> VILPNNDRHQITDTTNGHYAPVTYIQVEAPTGTFIASGVVVGKDTLLTNKHVVDATHGDPHALKAFPSAINQDNYPNGGFTAEQITKYSGEGDLAIVKFSPNEQNKHIGEVVKPATMSNNAETQVNQNITVTGYPGDKPVATMWESKGKITYLKGEAMQYDLSTTGGNSGSPVFNEKNEVIGIHWGGVPNEFNGAVFINENVRNFLKQNIEDINFANDDQPNNPDNP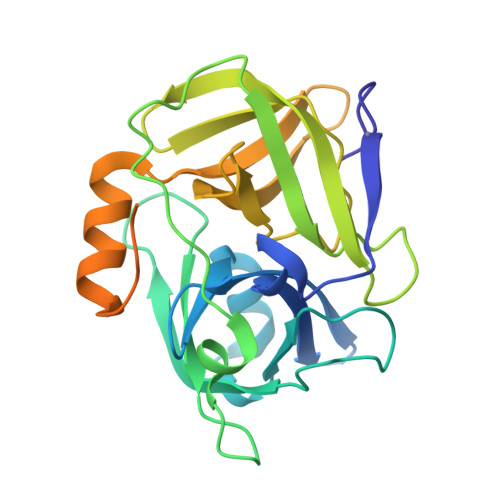DNPNNPDNPNNPDEPNNPDNPNNPDNPDNGDNNNSDNPDAA5-(4-methoxyphenyl)-N-[4-(4-methylpiperazin-1-yl)phenyl][1,2,4]triazolo[1,5-a]pyridin-2-amine | C24 H26 N6 O | 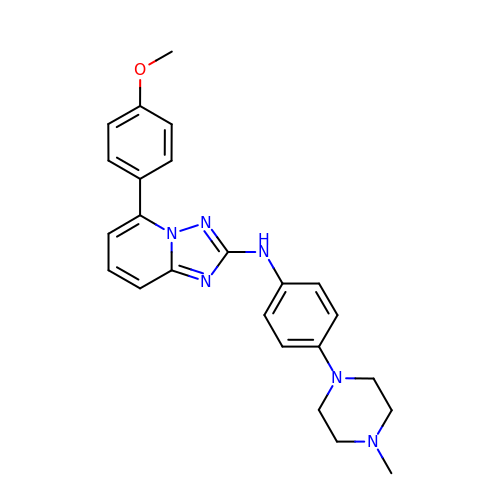DPVQBIWIVWTDRV-UHFFFAOYSA-N4-(1~{H}-indol-3-yl)butan-2-one | 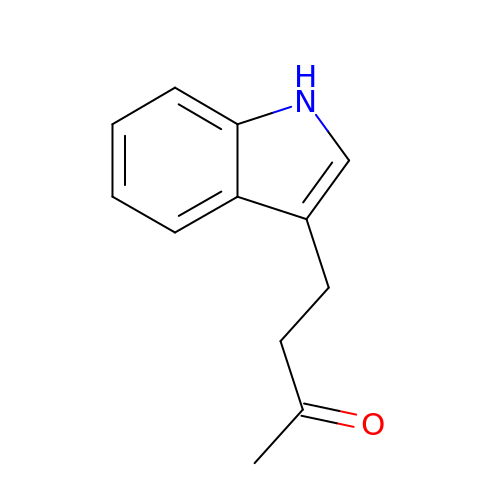C12 H13 N O | ZJCUUXGLZWBCIL-UHFFFAOYSA-N> ALLDETPLPPGSRLDVRAYTTVLHALSRAGRYERALELFAELRRQGVAPTVVTYNTLIDGL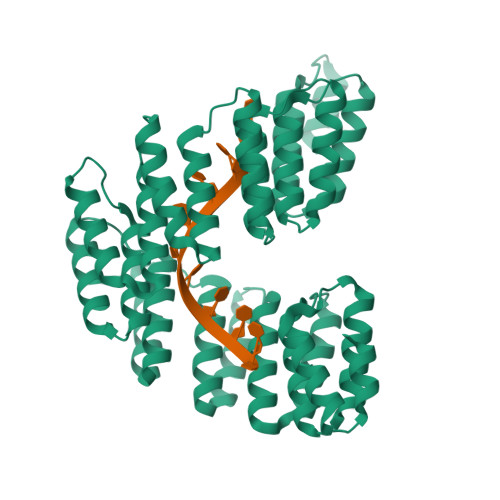CKAGKLDEALKLFEEMVEKGIKPDVVTYNTLIDGLCKAGKLDEALKLFEEMVEKGIKPDVVTYNTLIDGLCKAGKLDEALKLFEEMVEKGIKPDVVTYNTLIDGLCKAGKLDEALKLFEEMVEKGIKPDVVTYNTLIDGLCKAGKLDEALKLFEEMVEKGIKPDVVTYNTLIDGLCKAGKLDEALKLFEEMVEKGIKPDVVTYNTLIDGLCKAGKLDEALKLFEEMVEKGIKPDVVTYNTLIDGLCKAGKLDEALKLFEEMVEKGIKPDVVTYNTLIDGLCKAGKLDEALKLFEEMVEKGIKPDVVTYNTLIDGLCKAGKLDEALKLFEEMVEKGIKPDELTYRRVVESYCRAKRFEEARGFLSEVSETDLDFDKKALEAYIEDAQFGRLEHHHHHHHH>XLAAALMQ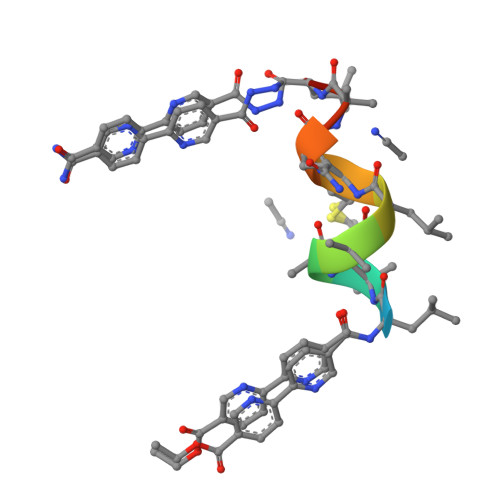ALX[2x]> MAYKPQ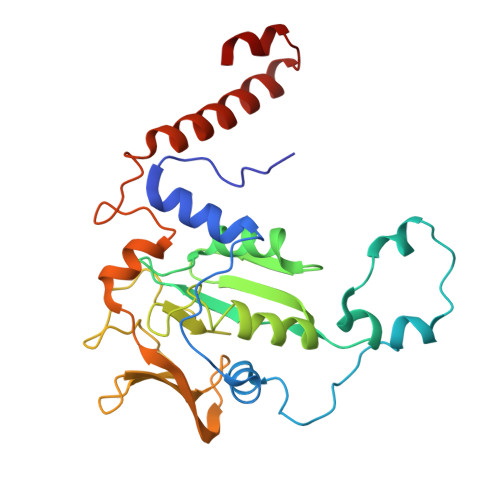FYPGETKIAQNRRNHMNPEVELEKLREIPDEDVVKIMGHRQPGEDYKTIHPPLEEMDLPDDYVRDLVEPINGAKEGHRIRYIQFADSMYFAPAQPYDRARTYMWRFRGVDTGTLSGRQVIEMRESDLEALSKNFLIDTAFFDPARCGIRGATVHGHSLRLDENGLMFDALQRYVYDEKTGHVVYVKDQVGRPLDEPVDVGELLPEEKLREITTIYRKDGVPMREDKELLTIVKRIHRARTLGGFCPTEDTFKQL> MILHALTQYYQRKAESDGGIAQEGFENKEIPFIIVIDKQGNFIQLEDTRELKVKKKVGRTFLVPKGLGRSGSKSYEVSNLLWDHYGYVLAYAGEKGQEQADKQHASFTAKVNELKQALPDDAGVTAVAAFLSSAEEKSKVMQAANWAECAKVKGCNLSFRLVDEAVDLVCQSKAVREYVSQANQTQSDNAQKGICLVTGKAAPIARLHNAVKGVNAKPAPFASVNLSAFESYGKEQGFAFPIGEQAMFEYTTALNTLLAGENRFRIGDVTTVCWGAKRTPLEESLASMINGGGKDKPDEHIDAVKTLYKSLYNGQYQKPDGKEKFYLLGLSPNSARIVVRFWHETTVAALSESIAAWYDDLQMVRGENSPYPEYMPLPRLLGNLVLDGKMENLPSDLIAQITDAALNNRVLPVSLLQAALRRNKAEQKITYGRASLLKAYINRAIRAGRLKNMKELTMGLDRNRQDIGYVLGRLFAVLEKIQAEANPGLNATIADRYFGSASSTPIAVFGTLMRLLPHHLNKLEFEGRAVQLQWEIRQILEHCQRFPNHLNLEQQGLFAIGYYHETQFLFTKDALKN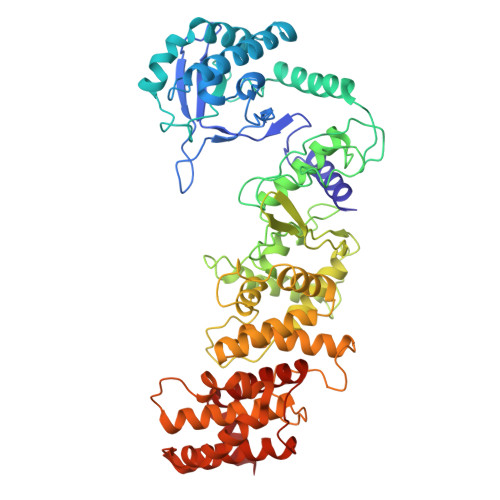LFNEA> GPMALTLVEQILAEFQLQEEDLKKVMRRMQKEMDRGLRLETHEEASVKMLPTYVRSTPEGSEVGDFLSLDLGGTNFRVMLVKVGEGEEGQWSVKTKHQMYSIPEDAMTGTAEMLFDYISECISDFLDKHQMKHKKLPLGFTFSFPVRHEDIDKGILLNWTKGFKASGAEGNNVVGLLRDAIKRRGDFEMDVVAMVNDTVATMISCYYEDHQCEVGMIVGTGCNACYMEEMQNVELVEGDEGRMCVNTEWGAFGDSGELDEFLLEYDRLVDESSANPGQQLYEKLIGGKYMGELVRLVLLRLVDE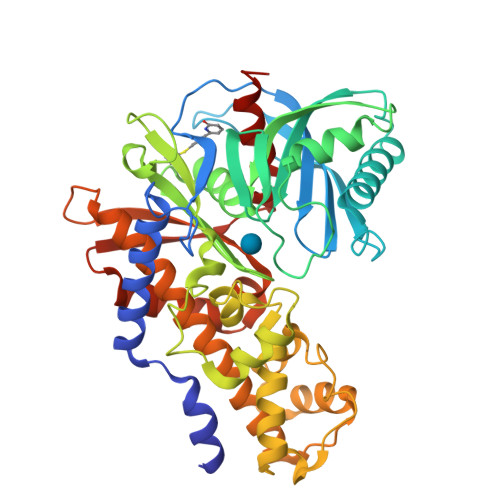NLLFHGEASEQLRTRGAFETRFVSQVESDTGDRKQIYNILSTLGLRPSTTDCDIVRRACESVSTRAAHMCSAGLAGVINRMRESRSEDVMRITVGVDGSVYKLHPSFKERFHASVRRLTPSCEITFIESEEGSGRGAALVSAVACKKACMLGQ3-BROMO-7-NITROINDAZOLE | C7 H4 Br N3 O2 | 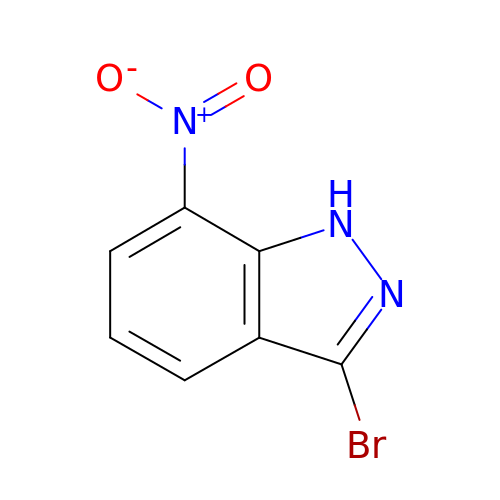NFSTZPMYAZRZPC-UHFFFAOYSA-N> IKPSNILPVTVYDQHGFRI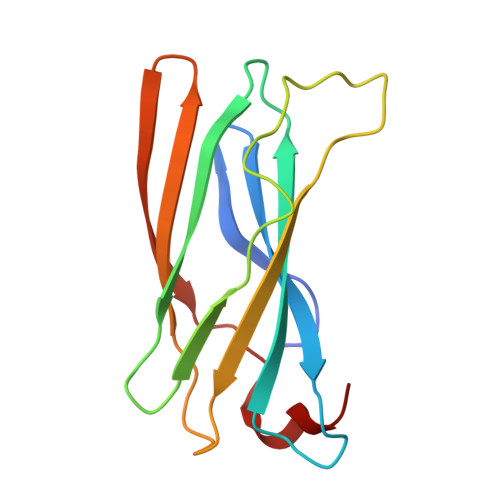LFHFARDPLPGRSDVLVVVVSMLSTAPQPIRNIVFQSAVPKVMKVKLQPPSGTELPAFNPIVHPSAITQVLLLANPQKEKVRLRYKLTFTMGDQTYNEMGDVDQFPPPETWGSL>[6x]MRIGYGEDSHRLEEGRPLYLCGLLIPSPVGALAHSDGDAAMHALTDALLSAYGLGDIGLLFPDTDPRWRGERSEVFLREAMRLVEARGAKLLQASLVLTLDRPKLGPHRK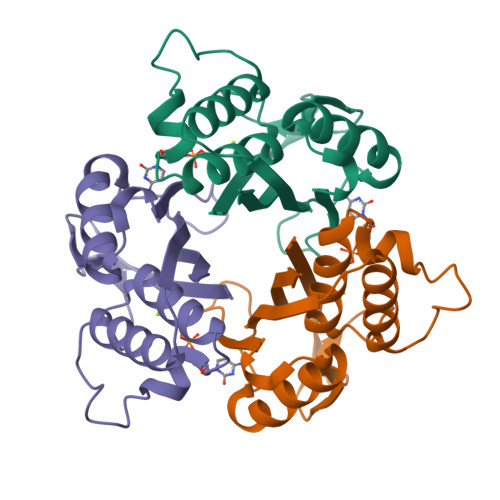ALVDSLSRLMRLPQDRIGLTFKTSEGLAPSHVQARAVVLLDG>MDDDGTGQKQIWRIEGSNKVPVDPATYGQFYGGDSYIILYNYRHGGRQGQIIYNWQGAQSTQDEVAASAILTAQLDEELGGTPVQSRVVQGKEPAHLMSLFGGKPMIIYKGGTSREGGQTAPASTRLFQVRANSAGATRAVEVLPKAGALNSNDAFVLKTPSAAYLWVGTGASEAEKTGAQELLRVLRAQPVQVAEGSEPDGFWEALGGKAAYRTSPRLKDKKMDAHPPRLFACSNKIGRFVIEEVPGELMQEDLATDDVMLLDTWDQVFVWVGKDSQEEEKTEALTSAKRYIETDPANRDRRTPIT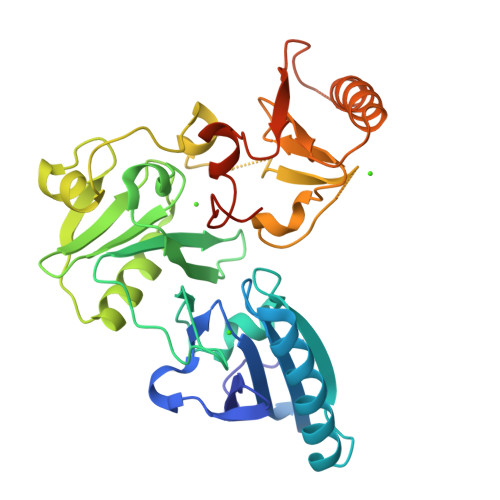VVKQGFEPPSFVGWFLGWDDDYWSVDPLDRAMAELAA[3x]> GAMGRSLLQHCKPFRGATKGCLRALAMKFKTTHAPPGDTLVHAGDLLTALYFISRGSIEILRGDVVVAILGKNDIFGEPLNLYARPGKS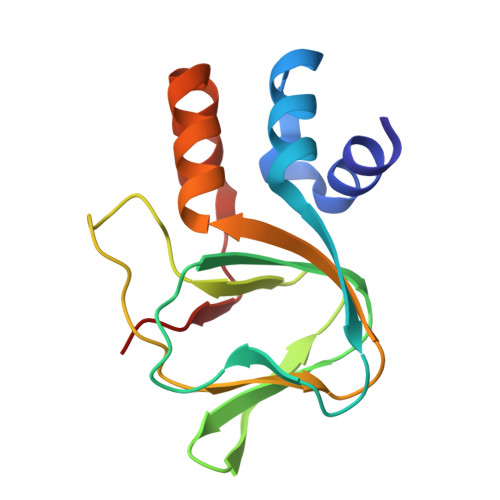NGDVRALTYCDLHKIHRDDLLEVLDMYPEFSDHFWSSLEITFNLRD> GPAKQYDSVECPFCDEVSKYEKLAKIGQGTFGEVFKARHRKTGQKVALKKVLMENEKE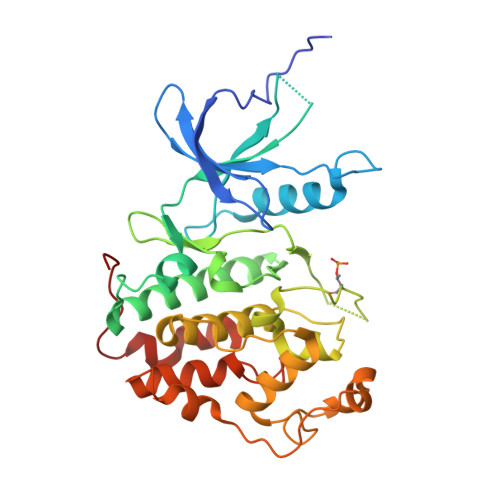GFPITALREIKILQLLKHENVVNLIEICRTKASPYNRCKASIYLVFDFCEHDLAGLLSNVLVKFTLSEIKRVMQMLLNGLYYIHRNKILHRDMKAANVLITRDGVLKLADFGLARAFSLAKNSQPNRYTNRVVTLWYRPPELLLGERDYGPPIDLWGAGCIMAEMWTRSPIMQGNTEQHQLALISQLCGSITPEVWPNVDNYELYEKLELVKGQKRKVKDRLKAYVRDPYALDLIDKLLVLDPAQRIDSDDALNHDFFWSDPMPSDLKGMLST>MNAIGNFLVGTPVFTIFIALALGYLLGKLKIGSFTLGATVGVLIVALLIGQLGVFPRDTCLGDIFFDFFMFAIGYRVGPSFISSMKKFGAKIVYATLIFLVSAFIVAYAAFKMFHIGPGIAAGIIAGGLTQSAVIGSSLETISKLPISDHLKTLYSNQIPIVYTLTYVFGTIGVLIFLRDIMPKLMHIDLKKQAVKTAKELDMIPVPVIVASTHFYTINDGSSLIGQTLGTVNTKFAKGLVAAGLNDSADMASVINAGDVLAISGGIDEIGRAVQEFNLLEVTGKTKAYVSKQVVLKKNFSADVLKNAQDKGVLVATLAGDVMDPAQFSTLKPAESVTLVGQKDAVSEVQSQLGRLRAAENIINYSWFALGIALSAALGIVGTKVSGVPIALGGGTASLIVGLVQSIYRDKHAHMDTIPDSLL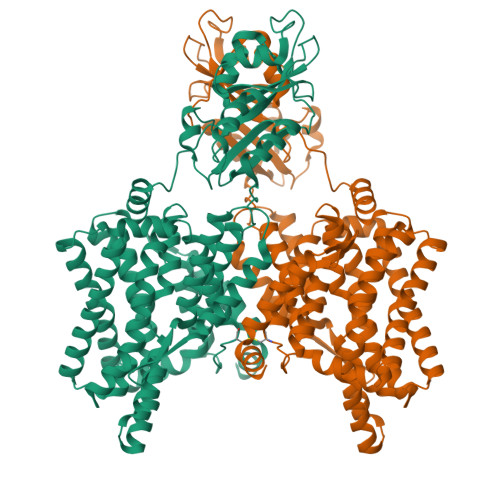EFFQSIGLNLFIATVGLSAAKTFISAIQSMGISVLLIGAVISILPHIITFVIAYYLMKMEPISIIGAQTGADTLSAALNDVSERVGSDASPFFAAAVAPAYAIGNIFLTLMGPIFIVLLS[2x]5-IODOURACIL | C4 H3 I N2 O2 | 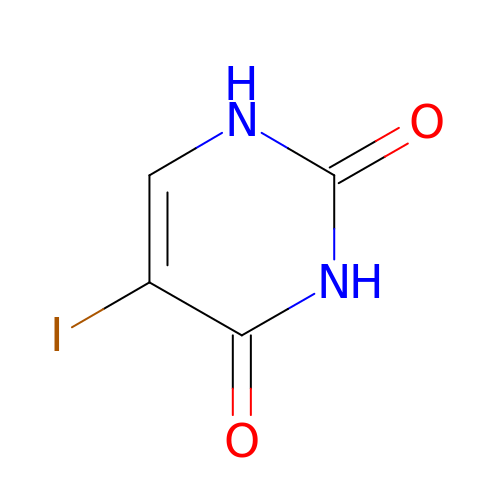KSNXJLQDQOIRIP-UHFFFAOYSA-N4-methyl-3-[4-(1-methylpiperidin-4-yl)phenyl]-5-(3,4,5-trimethoxyphenyl)pyridine 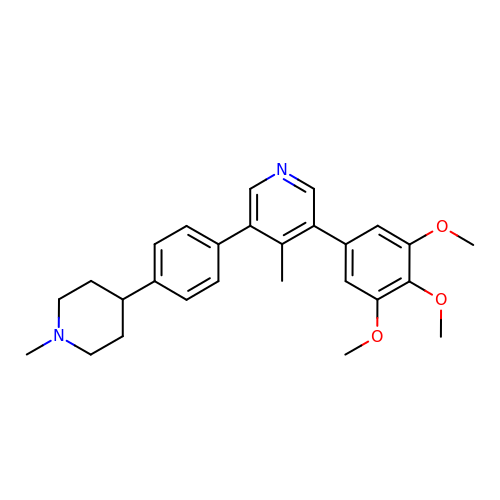| C27 H32 N2 O3 | CNEAZWBYXISKKK-UHFFFAOYSA-N> TQAEKTATDLPPGFSGKAGSVNATPGTKGLDGPTPLADGSFDATIFGPAKELKSADDILNVHRRNAKDPFAVGSVDAPLVITEFSDFECPFCARWSNQTEPMLMEEYVSKGLVRIEWNDLPVNGEHALAAAKAGR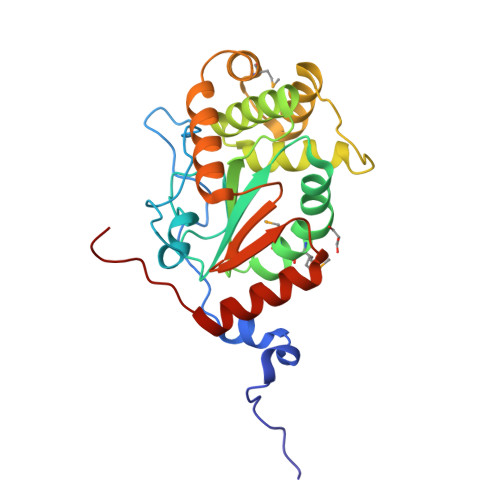AAAAQGKFDEFRKALFEASRNVSGHPNNTLKDFERFARNAGVKDMERFSREAQDSTYDEVLAKAADYAHGLGVSGTPAFVVGTQYISGAQPTEEFIKVIESELKKSPTFSTPSSH> ANPLYQKHIISINDLSRDDLNLVLATAAKLKANPQPELLKHKVIASCFFEASTRTRLSFETSMHRLGASVVGFSDSANTSLGKKGETLADTISVISTYVDAIVMRHPQEGAARLATEFSGNVPVLNAGDGSNQHPTQTLLDLFTIQETQGRL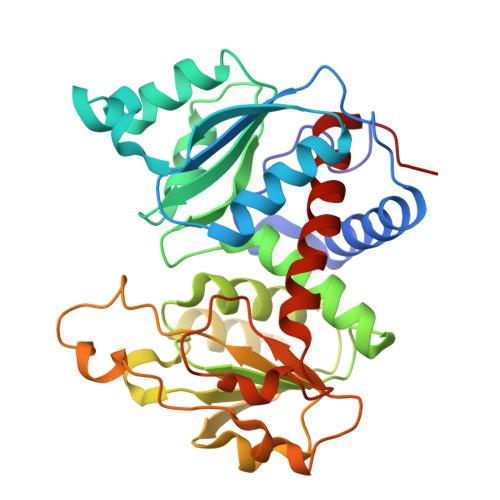DNLHVAMVGDLKYGRTVHSLTQALAKFDGNRFYFIAPDALAMPQYILDMLDEKGIAWSLHSSIEEVMAEVDILYMTRVQKERLAPSEYANVKAQFVLRASDLHNAKANMKVLHPLPRVDEIATDVDKTPHAWYFQQAGNGIFARQALLALVLNRDLVL> TRKLCSLDNGDCDQFCHE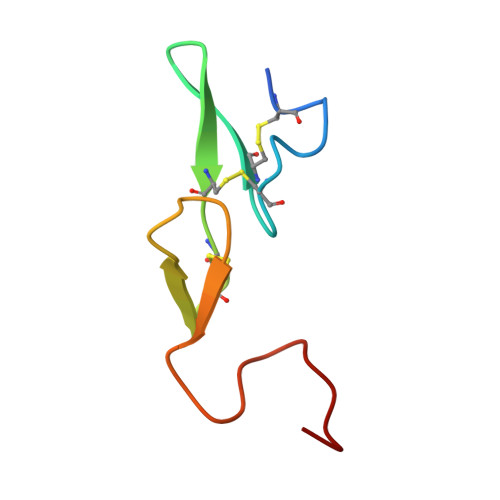EQNSVVCSCARGYTLADNGKACIPTGPYPCGKQTLE> MDPIRSFCGK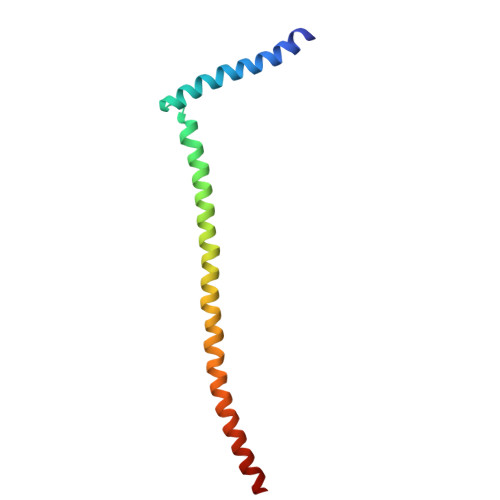LRSLASTLDCETARLQRALDGEESDFEDYPMRILYDLHSEVQTLKDDINILLDKARLENQEGIDFIKATKVLMEKNSMDIMKIREYFQKYG>[3x]QAQITGRPEWIWLALGTALMGLGTLYFLVKGMGVSDPDAKKFYAITTLVPAIAFTMYLSMLLGYGLTMVPFGGEQNPIYWARYADWLFTTPLLLLDLALLVDADQGTILALVGA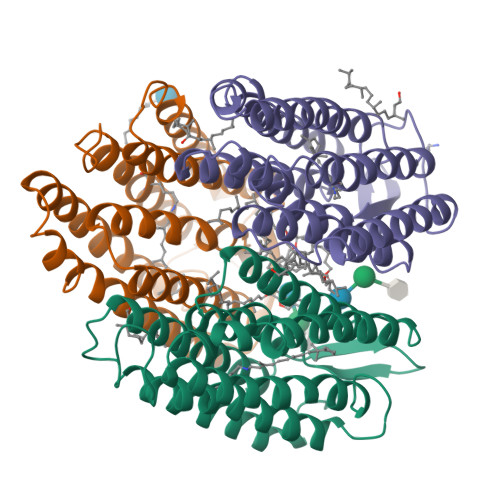DGIMIGTGLVGALTKVYSYRFVWWAISTAAMLYILYVLFFGFTSKAESMRPEVASTFKVLRNVTVVLWSAYPVVWLIGSEGAGIVPLNIETLLFMVLDVSAKVGFGLILLRSRAIFGEAEAPEPSADGAAATS> SNASETSGD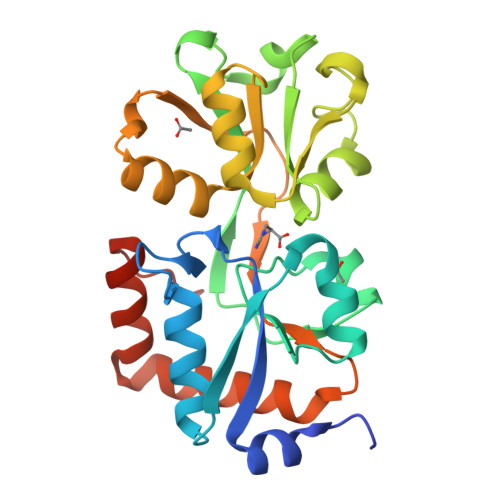NWSKYQSNKSITIGFDSTFVPMGFAQKDGSYAGFDIDLATAVFEKYGITVNWQPIDWDLKEAELTKGTIDLIWNGYSATDERREKVAFSNSYMKNEQVLVTKKSSGITTAKDMTGKTLGAQAGSSGYADFEANPEILKNIVANKEANQYQTFNEALIDLKNDRIDGLLIDRVYANYYLEAEGVLNDYNVFTVGLETEAFAVGSRKEDTTLVKKINEAFSSLYKDGKFQEISQKWFGEDVATKEVKEGQ>[2x]GPNCAPGQKVKLFRASEPILSVLMWGVNHTINELSNVPVPVMLMPDDFKAYSKIKVDNHLFNKENLPSRFKFKEYCPMVFRNLRERFGIDDQDYQNSVTRSAPINSDSQGRCGTRF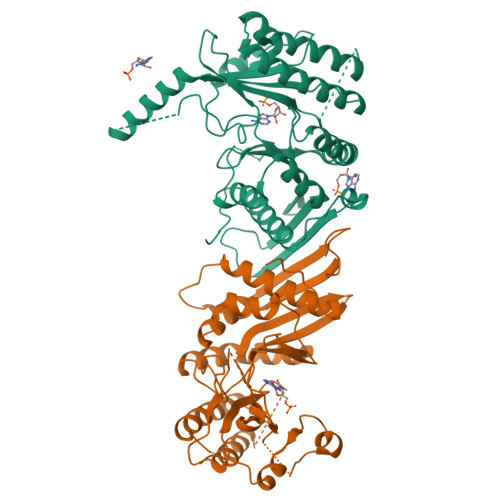LTTYDRRFVIKTVSSEDVAEMHNILKKYHQFIVECHGNTLLPQFLGMYRLTVDGVETYMVVTRNVFSHRLTVHRKYDLKGSTVAREASDKEKAKDLPTFKDNDFLNEGQKLHVGEESKKNFLEKLKRDVEFLAQLKIMDYSLLVGIHDVDRAEQEEMEVEERAEDEECENDGVGGNLLCSYGTPPDSPGNLLSFPRFFGPGEFDPSVDVYAMKSHESSPKKEVYFMAIADILTPYDTKKKAAHAAKTVKHGAGAEISTVNPEQYSKRFNEFMSNILT>[2x]GSGMSYAMCLNTFVLKKEVSETQHG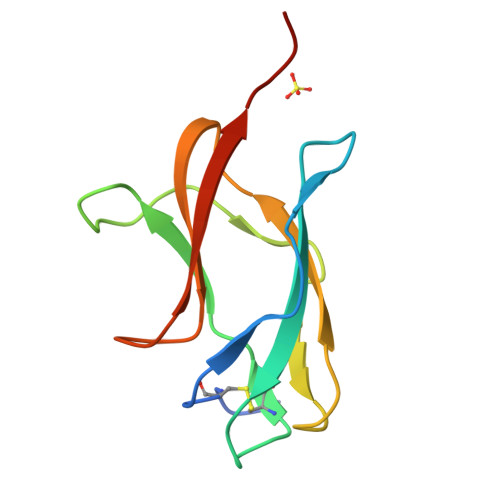TILIKVEYKGEDAPCKIPFSTEDGQGKAHNGRLITANPVVTKKEEPVNIEAEPPFGESNIVIGIGDKALKINWYRKGSSIGK>MVRGFYLRFGEGVSEEANRRALALAEALLRAPPPGLLDAVPAYGVLYLEYDPRRLSRGRLLRLLKGLPQERAEEGRVVEIPVRYDGEDLPEVASRLGLSLEAVKALHQKPLYRVYALGFTPGFPFLAEVEPALRLPRKPHPRPRVPAHAVAVAGVQTGIYPLPSPGGWNLLGTSLVAVYDPHRETPFLLRPGDRVRFLEAEGPTPPEPRPLELLPEEPRLPALLVEEPGLMDLVVDGGRFLGGHLGLARSGPLDAPSARLANRLVGNGAGAPLLEFAYKGPVLTALRDLVAAFAGYGFV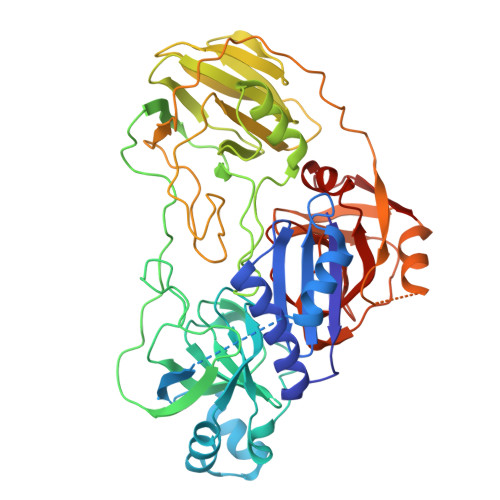ALLEGEEIPPGQSFLWPRGKTLRFRPRGPGVRGYLAVAGGLEVRPFLGSASPDLRGRIGRPLWAGDVLGLEALRPVRPGRAFPQRPLPEAFRLRLLPGPQFAGEAFRALCSGPFRVARADRVGVELLGPEVPGGEGLSEPTPLGGVQVPPSGRPLVLLADKGSLGGYAKPALVDPRDLWLLGQARPGVEIHFTSG[2x]>GPLGSGSGHLAIGSAATLGSGGMARGREPGGVGHVVAQVQSVDGNAQCCDCREPAPEWASINLGVTLCIQCSGIHRSLGVHFSKVRSLTLDSWEPELVKLMCELGNVIINQIYEARVEAMAVKKPGPSCSRQEKEAWIHAKYVEKKFLTKLPEIRGRRGGRGRPRGQPPVPPKPSIRPRPGDLRSKPEPPSEDLGSLHPGALLFRASGHPPSLPTMADALAHGADVNWVNGGQDNATPLIQATAANSLLACEFLLQNGANVNQADSAGRGPLHHATILGHTGLACLFLKRGADLGARDSEGRDPL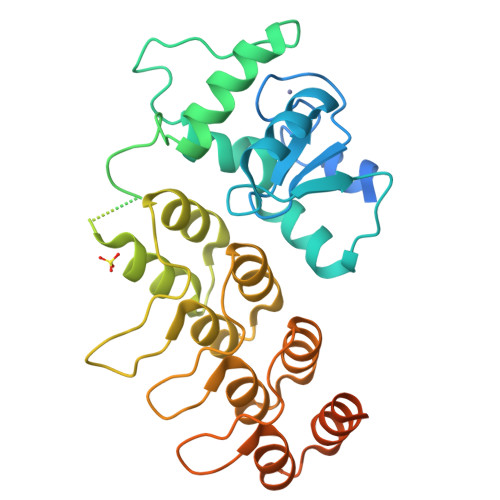TIAMETANADIVTLLRLAKMREAEAAQGQAGDETYLDIFRDFSLMASDDPEKLSRRSHDLHTL[2x]> MDDQLKQSALDFHEFPVPGKIQVSPTKPLATQRDLALAYSPGVAAPCLEIEKDPLKAYKYTARGNLVAVISNGTAVLGLGNIGALAGKPVMEGKGVLFKKFAGIDVFDIEVDELDPDKFIEVVAALEPTFGGINLEDIKAPECFYIEQKLRERMNIPVFHDDQHGTAIISTAAILNGLRVVEKNISDVRMVVSGAGAAAIACMNLLVALGLQKHNIVVCDSKGVIYQGREPNMAETKAAYAVVDDGKRTLDDVIEGADIFLGCSGPKVLTQEMVKKMARAPMILALANPEPEILPPLAKEVRPDAIICTGRSDYPNQVNNVLCFPFIFRGALDVGATAINEEMKLAAVRAIAELAHAEQSEVVASAYGDQDLSFGPEYIIPKPFDPRLIVKIAPAVAKAAMESGVATRPIADFDVYIDKLTEFVYKTNLFMKPIFSQARKAPKRVVLPEGEEARVLHATQELVTLGLAKPILIGRPNVIEMRIQKLGLQIKAGVDFEIVNNESDPRFKEYWTEYFQIMKRRGVTQEQAQRALISNPTVIGAIMVQRGEADAMICGTVGDYHEHFSVVKNVFGYRDGVHTAGAMNALLLPSGNTFIADTYVNDEPDAEELAEITLMAAETVRRFGIEPRVALLSHSNFGSSDCPSSSKMRQALELVRERAPELMIDGEMHGDAALVEAIRNDRMPDSSLKGSANILVMPNMEAARISYNLLRVSSSEGVTVGPVLMGVAKPVHVLTPIASVRRIVNMVALAVVEAQTQPL

While reducing NAD(P)+ to NAD(P)H, MEs catalyze the oxidative decarboxylation of the TCA cycle intermediate L-malate to produce the TCA carbon source pyruvate and a byproduct carbon dioxide (CO2) in the presence of divalent metal ions such as a magnesium (Mg2+) ion. The hybrid-type MEs consist of an N-terminal catalytic domain (ME domain) and a C-terminal activity regulating domain. The PTA domain does not possess an enzymatic activity of PTA but acts as an allosteric modulator of catalysis; that is, binding of some metabolites to the PTA domain increases or decreases the enzymatic activity. Binding of acetyl-CoA to the PTA domain is known to reduce the catalytic activity of several hybrid-type MEs.

To find the acetyl-CoA binding site of EcMaeB, we collected cryo-EM data of EcMaeBholo in the presence of acetyl-CoA (EcMaeBacetyl-CoA) and determined its structure at 2.03 Å resolution. This structure reveals that EcMaeBacetyl-CoA forms the V state as does EcMaeBholo. Acetyl-CoA molecules were located outside the apex of a triangle formed by the PTA domains. As a result, acetyl-CoA binds to the positively charged surface outside the PTA domain in EcMaeB. At the acetyl-CoA binding site of EcMaeB, the thioacetyl group of acetyl-CoA is inserted into the space created by the α4 and α5 helices and the loop region (V499–R506). Acetyl-CoA binds to EcMaeB mainly through interactions with three amino acids: R475, R482, and Y510. R475 forms a hydrogen bond with one of the carbonyl O atoms of the pantothenic acid moiety in acetyl-CoA. R482 forms a hydrogen bond with one of the phosphate groups of acetyl-CoA. The methyl group of the acetyl tail in acetyl-CoA shows a CH-π interaction with Y510. The α4 helix shifts to approach acetyl-CoA by 1.5 Å and the α5 helix moves away from acetyl-CoA by 1.4 Å.N-{4-4-(2,4-DIAMINO-6-OXO-1,6-DIHYDRO-PYRIMIDIN-5-YL)-1-(2,2,2-TRIFLUORO-1,1-DIHYDROXY-ETHYL)-BUT-2-YL-BENZOYL}-GAMMA-GLUTAMYL-GAMMA-GLUTAMYL-GLUTAMIC 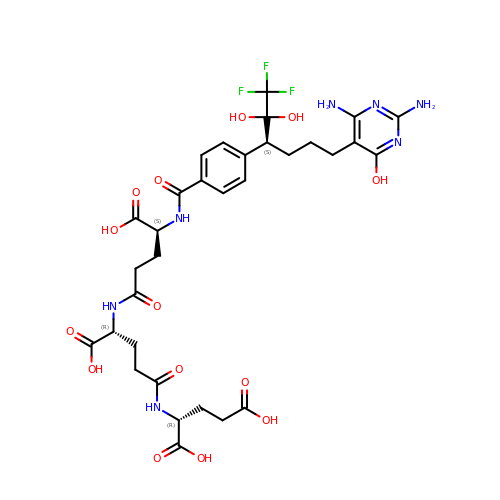ACID | C32 H40 F3 N7 O14 | DJAOVLPLLJHHPY-FVELJTHGSA-N6-({(3R,4R)-4-[4-(3-chloro-5-fluorophenoxy)butoxy]pyrrolidin-3-yl}methyl)-4-methylpyridin-2-amine | C21 H27 Cl F N3 O2 | 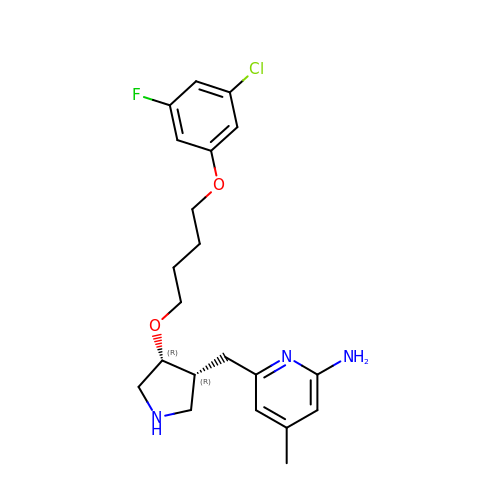AXHBVFDWXKWFTE-QRWLVFNGSA-N>MGHHHHHHHHHHSSGHIEGRHMK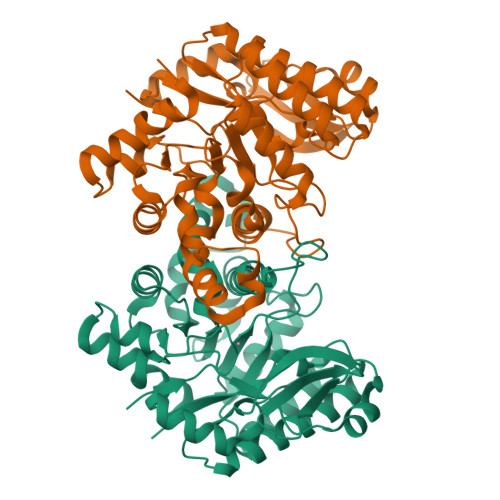KPRIDMHSHFFPRISEQEAAKFDANHAPWLQVSAKGDTGSIMMGKNNFRPVYQALWDPAFRIEEMDAQGVDVQVTCATPVMFGYTWEANKAAQWAERMNDFALEFAAANPQRIKVLAQVPLQDLDLACKEASRAVAAGHLGIQIGNHLGDKDLDDATLEAFLTHCANEDIPILVHPWDMMGGQRMKKWMLPWLVAMPAETQLAILSLILSGAFERIPKSLKICFGHGGGSFAFLLGRVDNAWRHRDIVREDCPRPPSEYVDRFFVDSAVFNPGALELLVSVMGEDRVMLGSDYPFPLGEQKIGGLVLSSNLGESAKDKIISGNASKFFNINV[2x]>MIPAHVPADRVVDFDIFNPPGVEQDYFAAWKTLLDGPGLVWSTANGGHWIAARGDVVRELWGDAERLSSQCLAVTPGLGKVMQFIPLQQDGAEHKAFRTPVMKGLASRFVVALEPKVQAVARKLMESLRPRGSCDFVSDFAEILPLNIFLTLIDVPLEDRPRLRQLGVQLTRPDGSMTVEQLKQAADDYLWPFIEKRMAQPGDDLFSRILSEPVGGRPWTVDEARRMCRNLLFGGLDTVAAMIGMVALHLARHPEDQRLLRERPDLIPAAADELMRRYPTVAVSRNAVADVDADGVTIRKGDLVYLPSVL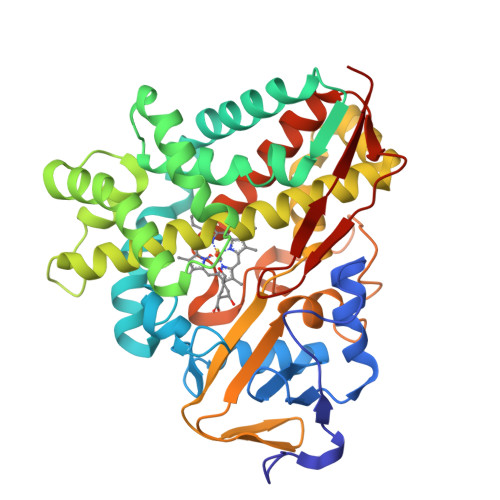HNLDPASFEAPEEVRFDRGLAPIRHTTMGVGAHRCVGAGLARMEVIVFLREWLGGMPEFALAPDKAVTMKGGNVGACTALPLVWRA[3x]> MSVTIDHTTENAAPAQAAVSDRAWALFRALDGKGLVPDGYVEGWKKTFEEDFSPRRGAELVARAWTDPEFRQLLL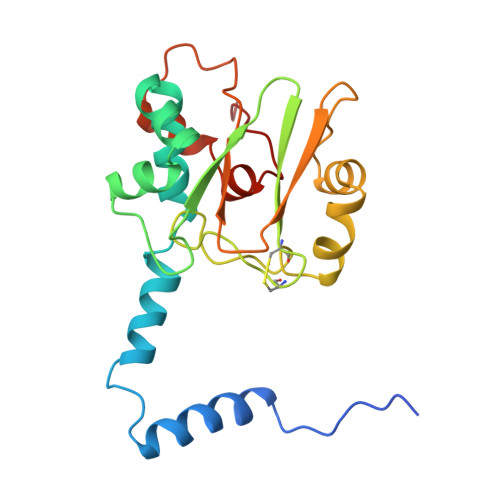TDGTAAVAQYGYLGPQGEYIVAVEDTPTLKNVIVCSLCSCTAWPILGLPPTWYKSFEYRARVVREPRKVLSEMGTEIASDIEIRVYDTTAETRYMVLPQRPAGTEGWSQEQLQEIVTKDCLIGVAIPQVPTV> HHMDEEYDVIVLGTGLTECILSGIMSVNGKKVLHMDRNPYYGGESSSITPLEELYKRFQLLEGPPETMGRGRDWNVDLIPKFLMANGQLVKMLLYTEVTRYLDFKVVEGSFVYKGGKIYKVPSTETEALASNLMGMFEKRRFRKFLVFVANFDENDPKTFEGVDPQNTSMRDVYRKFDLGQDVIDFTGHALALYRTDDYLDQPCLETINRIKLYSESLARYGKSPYLYPLYGLGELPQGFARLSAIYGGTYMLNKPVDDIIMENGKVVGVKSEGEVARCKQLICDPSYVPDRVRKAGQVIRIICILSHPIKNTNDANSCQIIIPQNQVNRK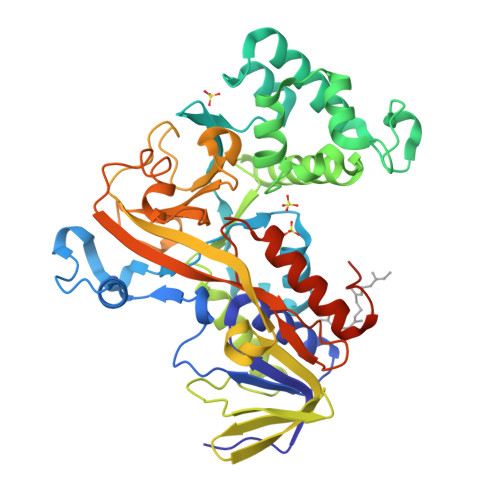SDIYVCMISYAHNVAAQGKYIAIASTTVETTDPEKEVEPALELLEPIDQKFVAISDLYEPIDDGSESQVFCSCSYDATTHFETTCNDIKDIYKRMAGSAFDFENMKRKQNDVFGEADQ> GDRSIEISIRVDDFTKTGEAVRYE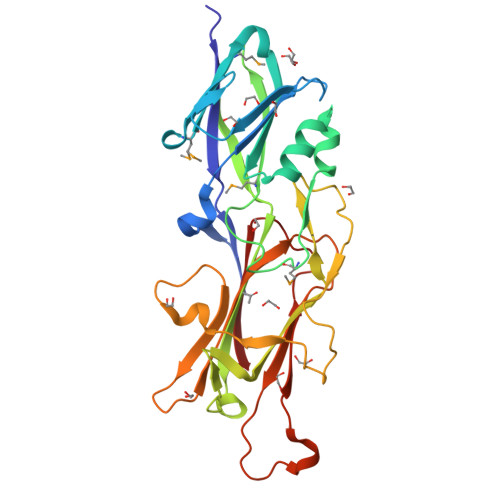RNQGSAAERLITNLYLLLFDQSGANPAKYYITGNTFTGGTWLPDDMKVKLDMTQSEAGERKVYVVANVDNAVKTALDAVANESDLQTVKRTTAMPWSTDIASPFLMSGNKTHDFLANRLLDNVPLVRAIAKVELNISLSEKFQIVPIIVNGSLSEFKFRYVNFDKETYVVKPTTKPDNLISSANGVWPQITDWTVWGASLNTSPAPDAGTGYTLDANGKVTALRIVTYLNERDSKGATVEVALPRVDDGTLPPPEFGPELYRLPLPDKILRNHWYKYEVEI>AAMEVIREQEFVNQYHYDARNLEWEEENGTPKTNFEVTFQLANRDEAAKVTSIVAVLQFVIVRDEFVISGVISQMAHIQGRLINEPSEFSQDEVENLAAPLLEI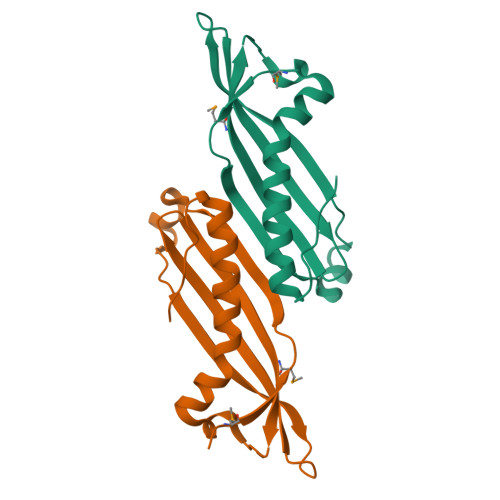VKRLTYEVTEIALDRPGVTLEFNS[4x]> GASGDLYEVERIVDKRKNKKGKWE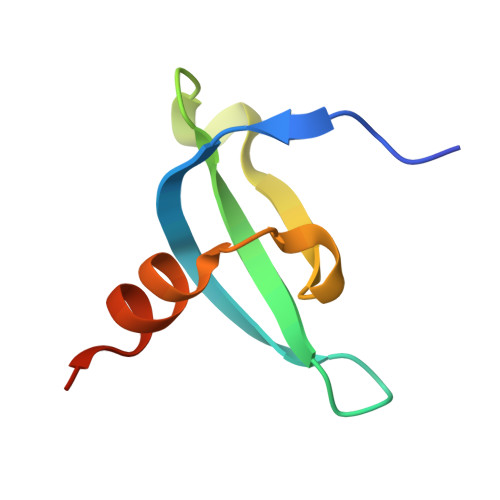YLIRWKGYGSTEDTWEPEHHLLHCEEFIDEFNGLHMSK>GAMDPEFMELRVGNRYRLGRKIGSGSFGDIYLGTDIAAGEEVAIKLECVKTKHPQLHIESKIYKMMQGGVGIPTIRWCGAEGDYNVMVMELLGPSLEDLFNFCSRKFSLKTVLLLADQMISRIEYIHSKNFIHRDVKPDNFLMGLGKKGNLVYIIDFGLAKKYRDARTHQHIPYRENKNLTGTARYASINTHLGIEQSRRDDLESLGYVLMYFNLGSLPWQGLKAATKRQKYERISEKKMSTPIEVLCKGYPSEFATYLNFCRSLRFDDKPDYSYLRQLFRNLFHRQGFSYDYVF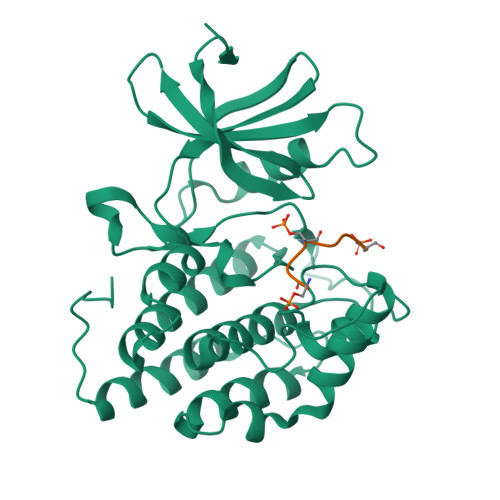DWNMLK[2x];>GKAESVASLTSQCSYA[2x]>TPEMPVLENRAAQGDITAPGGARRLTGDQTAALRDSLSDKPAKNIILLIGDGMGDSEITAARNYAEGAGGFFKGIDALPLTGQYTHYALNKKTGKPDYVTDSAASATAWSTGVKTYNGALGVDIHEKDHPTILEMAKAAGLATGNVSTAELQDATPAALVAHVTSRKCYGPSATSEKCPGNALEKGGKGSITEQLLNARADVTLGGGAKTFAETATAGEWQGKTLREQAQARGYQLVSDAASLNSVTEANQQKPLLGLFADGNMPVRWLGPKATYHGNIDKPAVTCTPNPQRNDSVPTLAQMTDKAIELLSKNEKGFFLQVEG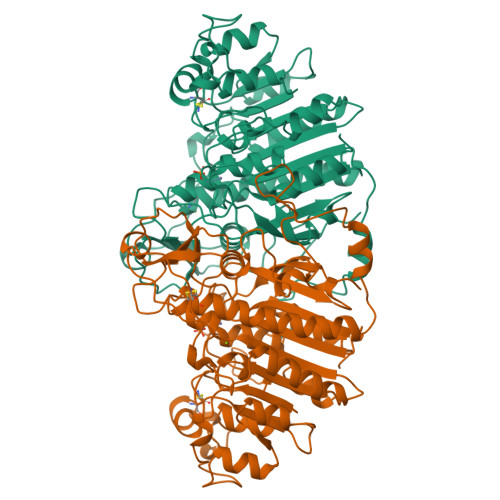ASIDKQDHAANPCGQIGETVDLDEAVQRALEFAKKEGNTLVIVTADHAHASQIVAPDTKAPGLTQALNTKDGAVMVMSYGNSEEDSQENTGSQLRIAAYGPHAANVVGLTDQTDLFYTMKAALGLK[2x]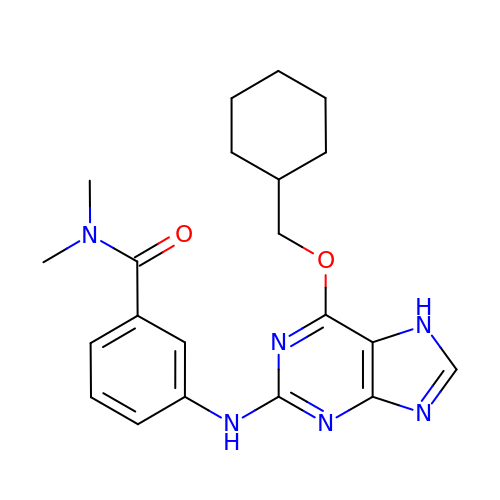3-[[6-(cyclohexylmethoxy)-7~{H}-purin-2-yl]amino]-~{N},~{N}-dimethyl-benzamide | C21 H26 N6 O2 | HZNQONMMEIJNNU-UHFFFAOYSA-N Here we demonstrate that HSL1 binds IDA/IDL peptides with high, and CLE peptides with lower affinity, respectively. Ligand sensing capability and receptor activation of HSL1 require a SERK co-receptor kinase. Crystal structures with IDA/IDLs or with CLE9 reveal that HSL1-SERK1 complex recognizes the entire IDA/IDL signaling peptide, while only parts of CLE9 are bound to the receptor. Our work reveals that HSL1 is a receptor for IDA/IDL signaling peptides.

The vastly different binding affinities between IDA/IDLs vs. CLE9 to HSL1 prompted us to determine co-crystal structures of four HSL1-IDA/IDL-SERK1 ternary complexes with: IDA, IDL1, IDL2, and IDL3 (at 2.31 Å, 2.38 Å, 2.20 Å, and 2.70 Å, respectively) and the HSL1-CLE9-SERK1 complex at 2.87 Å. Superposition of the four crystal structures yielded an R.M.S.D of ~0.6 Å comparing 590 Cα atom pairs, with IDL peptides perfectly aligning to each other. Given the high structural similarity among all IDA/IDL ternary complexes, we subsequently used the HSL1-IDA-SERK1 complex to further analyze the distinct ligand recognition mechanism between the IDA/IDLs and CLE peptide families. We first validated our HSL1-IDA-SERK1 structural model, by mutating key amino acids in the HSL1 ligand-binding surface and its interface with SERK1. Size-exclusion chromatography experiments of HSL1 mutants: HSL1Y261AR402A (ligand pocket) and HSL1N543AY544AN566A (receptor-co-receptor zipper-like interface), disrupted the formation of the ternary complex. The IDA core motif contains three conserved amino acids (Ser62IDA, Hyp64IDA, and Ser65IDA) that are specifically recognized by the receptor through a network of direct and water-mediated hydrogen bonds that anchor the peptide to the receptor. Removal of the hydroxyl group of the central Pro64 in IDA results in the loss of binding to HSL1 and disrupts the formation of the ternary complex. His68IDA acts as a bridging point between HSL1 and the SERK1 co-receptor, establishing hydrogen-bonding contacts with Glu376 in HSL1 and with the Asp51 in SERK1. To assess the contribution of the C-terminal region of IDA to HSL1 binding and co-receptor sensing, we engineered a Lys66/Arg67/His68→Ala mutant and we tested its efficiency in binding assays. The triple IDA mutant showed ~15 fold reduced binding affinity to HSL1 and a ~30-fold Kd reduction in the presence of the co-receptor compared to the wild-type peptide. The co-receptor SERK1 interacts with the C-terminal region of the different IDA/IDL peptides (residues 68-69 in IDA), completing the peptide-binding pocket using its N-terminal loop region.

>GSSMDNQDGFILQQVKLSLDDPDSYLSSWNSNDASPCRWSGVSCAGDFSSVTSVDLSSANLAGPFPSVICRLSNLAHLSLYNNSINSTLPLNIAACKSLQTLDLSQNLLTGELPQTLADIPTLVHLDLTGNNFSGDIPASFGKFENLEVLSLVYNLLDGTIPPFLGNISTLKMLNLSYNPFSPSRIPPEFGNLTNLEVMWLTECHLVGQIPDSLGQLSKLVDLDLALNDLVGHIPPSLGGLTNVVQIELYNNSLTGEIPPELGNLKSLRLLDASMNQLTGKIPDELCRVPLESLNLYENNLEGELPASIALSPNLYEIRIFGNRLTGGLPKDLGLNSPLRWLDVSENEFSGDLPADLCAKGELEELLIIHNSFSGVIPESLADCRSLTRIRLAYNRFSGSVPTGFWGLPHVNLLELVNNSFSGEISKSIGGASNLSLLILSNNEFTGSLPEEIGSLDNLNQLSASGNKFSGSLPDSLMSLGELGTLDLHGNQFSGELTSGIKSWKKLNELNLADNEFTGKIPDEIGSLSVLNYLDLSGNMFSGKIPVSLQSLKLNQLNLSYNRLSGDLPPSLAKDMYKNSFIGNPGLCGDIKGLCGSENEAKKRGYVLEGSENLYFQ[2x];>GSSMASANLEGDALHTLRVTLVDPNNVLQSWDPTLVNPCTWFHVTCNNENSVIRVDLGNAELSGHLVPELGVLKNLQYLELYSNNITGPIPSNLGNLTNLVSLDLYLNSFSGPIPESLGKLSKLRFLRLNNNSLTGSIPMSLTNITTLQVLDLSNNRLSGSVPDNGSFSLFTPISFANNLDLCGPVTSHPCPLEGSLENLYFQ[2x];>YVPIPPSAPSKRHN[2x]>[8x]FNCTSSSATVHWLGDKPTYHAGVTFGLPWPQGKYRP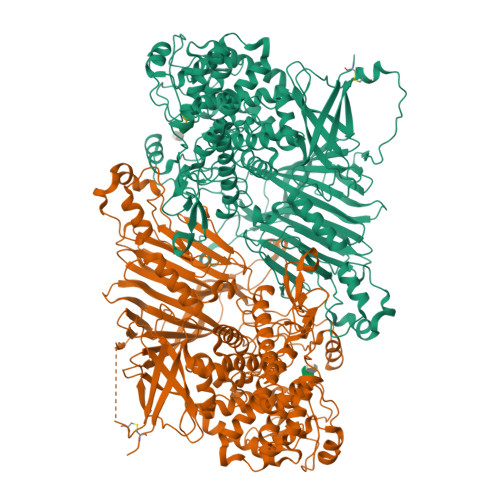QETSFSLTGDTEDKSELQSWATGYWADGSLKWTAHAIAESNQIYDQYTVTASSLGCVKSSSSSSESSAPNSSIVVTDNSDALTVNTGEVAVSFPKGGNVIIGDIKTKSGKVIGANGRLVLQSQDSVPDNFDNRANSPIQYSNFDGNINEVFVNQTSARTLVTVRGNHTVTDGTDHDPWLPFVVRFYLYANSATIKVMHSIVFDGDENDFITGLGIRFDVPLKGEEYYDRHIRFAGVDGGIFNEAVQGITGLRRDPGEEIRAAQFAGQKLADTETWEPRVSTRLKWIPTWADYGLTQLTADGFGLKKRTKAGQSWVNIPSGTRAEGLAYLGGATQGGLAVGLRDFWKRYPVGLDISNAASDTGELTLWLYSPAAEPLDLRPFHDGLGQDGYEDQLDALEITYEDWEPGFDTPYGIARTSEVYLFAFDQTPTSDKLASLTAYMNDPPVLVAEPKYIHETQALGEYWALPGSASPAAATLEDRLQFIFDFYKGQIEQRRWYGFLDYGDFMHTYDPDRHTWRYDVGGYAWDNSELSPDLFFWLYFLRTGSKDAYRFAEALTRHTGEVDVYHIGDWKGLGTRHGVQHWSDSAKQARISQPQYRKYFFYLSGGDERVGELLEELLDTDKTYGELDPQRKVRTDGWEPSPNSTVSFGLGTDWSGLAAGWLIEWERRGPRWEEAKTKLTNTIAGIANLTNGFVTGSGLYDPVTWTLGPPPSDPGNRGNVSISHLNAVFGLPEVVSEAIAYLADDIPKGFKQAWLDYCYYYHASASEQKDRYGVSFSKISLLQAHSRLAAYAAYETKNKTLALRAWKDFYASDGLLPDAPWNITHVDGSDVLVPVDEAAWLATNDIAQYGLAVIQNLAYVSDSLDDYQS> TISVRVTTMDAELEFAIQPNTTGKQLFDQVVKTIGLREVWFFGLQYQDTKGFSTWLKLNKKVTAQDVRKESPLLFKFRAKFYPEDVSEELIQDITQRLFFLQVKEGILNDDIYCPPETAVLLASYAVQSKYGDFNKEVHKSGYLAGDKLLPQRVLEQHKLNKDQWEERIQVWHEEHRGMLREDAVLEYLKIAQDLEMYGVNYFSIKN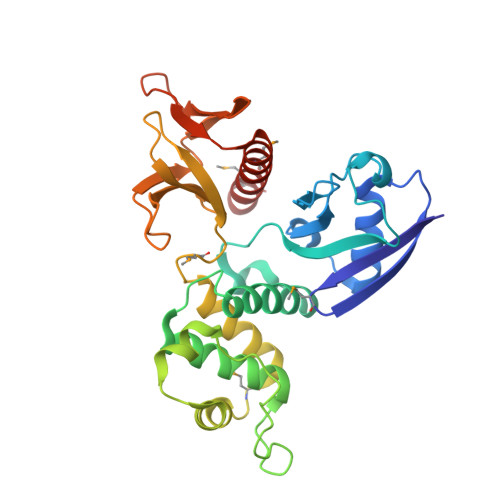KKGSELWLGVDALGLNIYEQNDRLTPKIGFPWSEIRNISFNDKKFVIKPIDKKAPDFVFYAPRLRINKRILALCMGNHELYMRRRKP>[2x]GGSVIVIDS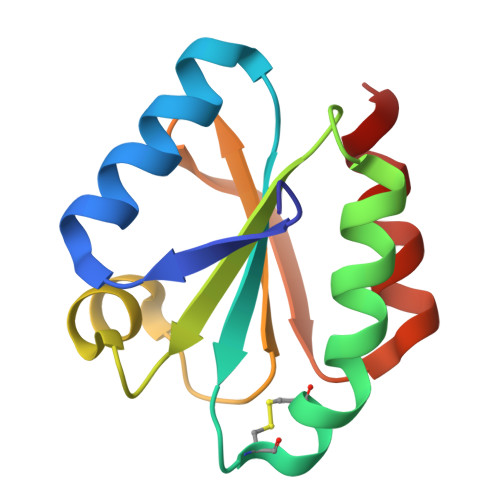KAAWDAQLAKGKEEHKPIVVDFTATWCGPCKMIAPLFETLSNDYAGKVIFLKVDVDAVAAVAEAAGITAMPTFHVYKDGVKADDLVGASQDKLKALVAKHAAA PF-3758309 | C25 H30 N8 O S | 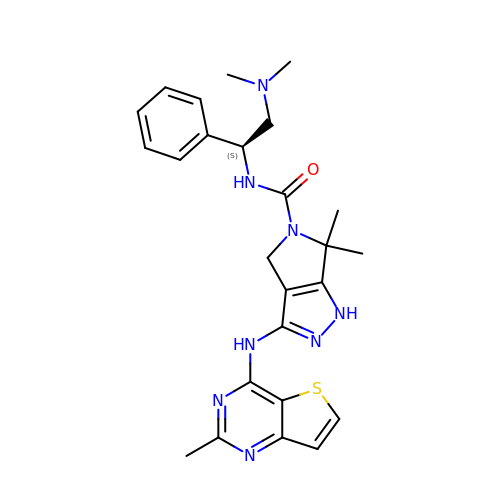AYCPARAPKDAOEN-LJQANCHMSA-N>[4x]AEAGITGTWYNQLGSTFIVTAGADGALTGTYESAVGNAESRYVLTGRYDSAP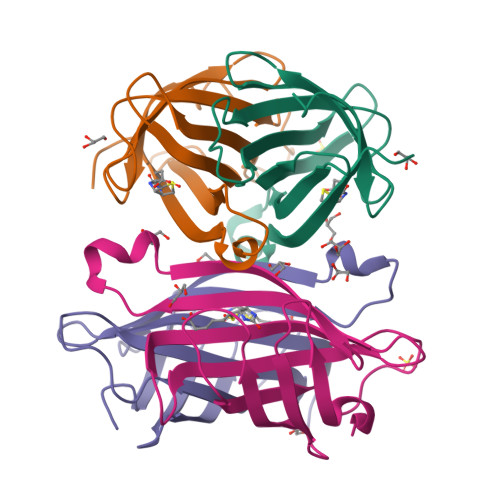ATDGSGTALGWTVAWKNNYRNAHSATTWSGQYVGGAEARINTQWLLTSGTTEANAWKSTLVGHDTFTKVKPSAAS>QPAPAWTTFRVGLFCGIFIVLNITLVLAAVFKLETDRSIWPLIRIYRGGFLLIEFLFLLGINTYGWRQAGVNHVLIFELNPRSNLSHQHLFEIAGFLGILWCLSLLACFFAPISVIPT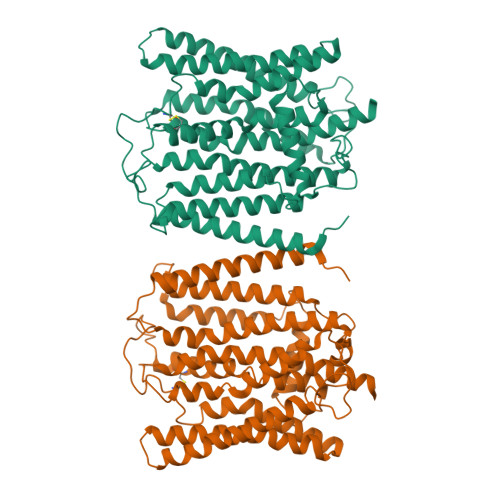YVYPLALYGFMVFFLINPTKTFYYKSRFWLLKLLFRVFTAPFHKVGFADFWLADQLNSLSVILMDLEYMICFYSLELKWDESKGLLPNNSEESGICHKYTYGVRAIVQCIPAWLRFIQCLRRYRDTKRAFPHLVNAGKYSTTFFMVTFAALYSTHKERGHSDTMVFFYLWIVFYIISSCYTLIWDLKMDWGLFDKNAGENTFLREEIVYPQKAYYYCAIIEDVILRFAWTIQISITSTTLLPHSGDIIATVFAPLEVFRRFVWNFFRLENEHLNNCGE[2x]> GHMVEIGELAPDFELPDTELKKVKLSALKGKVVVLAFYPAAFTQVCTKEMCTFRDSMAKFNQVNAVVLGISVDPPFSNKAFKEHNKLNFTI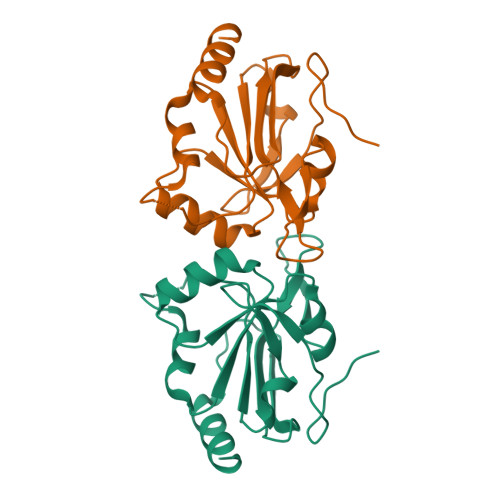LSDYNREVVKKYNVAWEFPALPGYVLAKRAVFVIDKEGKVRYKWVSDDPTKEPPYDEIEKVVKSLS>[2x]MDFLRNLFSQTLSLGSQKERLLDELTLEGVARYMQSERCRRVICLVGAGISTSAGIPDFRSPSTGLYDNLEKYHLPYPEAIFEISYFKKHPEPFFALAKELYPGQFKPTICHYFMRLLKDKGLLLRCYTQNIDTLERIAGLEQEDLVEAHGTFYTSHCVSASCRHEYPLSWMKEKIFSEVTPKCEDCQSLVKPDIVFFGESLPARFFSCMQSDFLKVDLLLVMGTSLQVQPFASLISKAPLST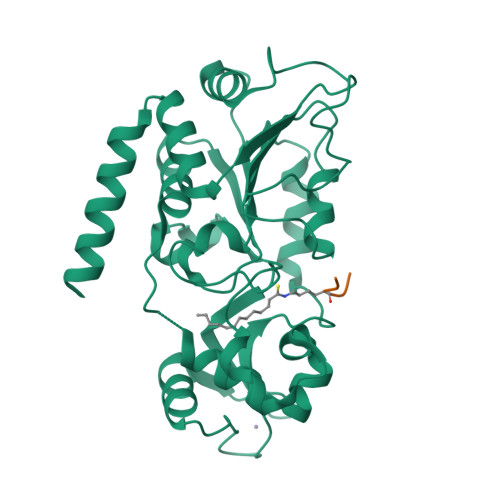PRLLINKEKAGQSDPFLGMIMGLGGGMDFDSKKAYRDVAWLGECDQGCLALAELLGWKKELEDLVRREHASIDAQS;>[2x]PKKTG> EWEALEKKL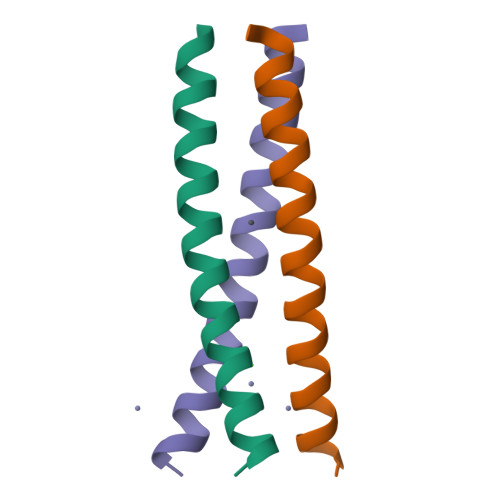AALESKCQALEKKLQALEKKHEALEHG>[2x]MSGETTRLTEPQLRELAARGAAELDGATATDMLRWTDETFGDIGGAGGGVSGHRGWTTCNYVVASNMADAVLVDLAAKVRPGVPVIFLDTGYHFVETIGTRDAIESVYDVRVLNVTPEHTVAEQDEL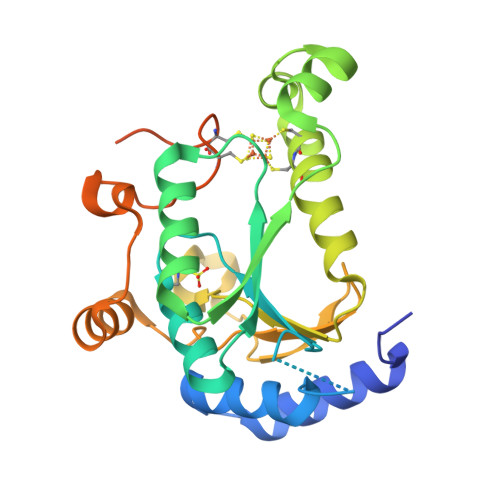LGKDLFARNPHECCRLRKVVPLGKTLRGYSAWVTGLRRVDAPTRANAPLVSFDETFKLVKVNPLAAWTDQDVQEYIADNDVLVNPLVREGYPSIGCAPCTAKPAEGADPRSGRWQGLAKTECGLHASLEHHHHHH>SHMQSDILEMVARGWKYFSGNFYYFSRTPKTWYSAEQFCISRKAHLTSVSSESEQKFLYKAADGIPHWIGLTKAGSEGDWYWVDQTSFNKEQSRRFWIPGEPNNAGNNEHCANIRVSALKSWNDGPCDNTFLFICKRPYVQTTEGTWSHPQFEK[2x]

Langerin, a member of the C-type lectin (CTL) superfamily, is a Ca2+-dependent carbohydrate-binding protein. This receptor is primarily expressed on Langerhans cells, antigen-presenting cells residing in the epidermis of the skin, where it plays a crucial role in various biological processes, in particular, in initiating the innate immune response. The canonical carbohydrate-binding site of CTLs features a long loop where the EPN (Glu-Pro-Asn) motif, responsible for its mannose specificity, is located. The recognition of the cofactor Ca2+ by langerin is tightly coupled to its life cycle as an endocytic and recycling receptor.

To further elucidate the structural basis of Ca2+ competition, we conducted X-ray crystallographic studies. The central proline in the EPN motif is crucial for the Ca2+ coordination. In this structure, Pro289 remains in the cis conformation while the long loop shows significant mobility, as indicated by the missing electron density, similar to the inhibitor-bound structure. This observation is consistent with previous NMR results showing 75 ± 10% of the central proline adopts the cis conformation in Ca2+-free human langerin. The pronounced long loop conformational differences between Ca2+-bound and unbound states highlight the sensitivity of the long loop to Ca2+. (D) Superposition of the four chains from both structures highlights marked differences in the long loop conformation, with only minor variability in the short loop. A similar mechanism has been described for another CTL, DC-SIGNR, where the loop adjacent to its secondary Ca2+ site shifts between open and closed states depending on Ca2+ binding. Therefore, it remains unclear whether the long loop structural rearrangement upon inhibitor binding is driven either by an induced fit mechanism, conformational selection, or a combination of both. X-ray crystallography revealed the binding site of inhibitor 3 and the long loop sensitivity toward Ca2+. The results highlight the long loop as a potential structural switch and offer a design strategy of future langerin and other CTL inhibitors.> MKSLGRHLVAEFYECDREVLDNVQLIEQEMKQAAYESGATIVTSTF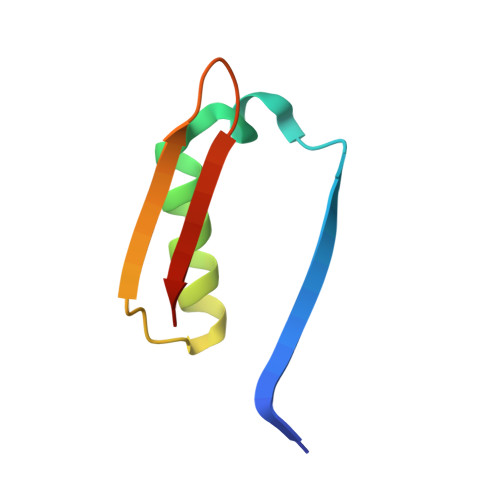HRFLPYGVSGVVVISE>[6x]MKDILEKLEERRAQARLGGGEKRLEAQHKRGKLTARERIELLLDHGSFEEFDMFVQHRSTDFGMEKQKIPGDGVVTGWGTVNGRTVFLFSKDFTVFGGSSSEAHAAKIVKVQDMALKMRAPIIGIFDAGGARIQEGVAALGGHGEVFRRNVAASGVIPQISVIMGPCAGGDVYSPAMTDFIFMVRDTSYMFVTGPDVVKTVTNEVVTAEELGGAKVHTSKSSIADGSFENDVEAILQIRRLLDFLPANNIEGVPEIESFDDVNRLDKSLDTLIPDNPNKPYDMGELIRRVVDEGDFFEIQAAYARNIITGFGRVEGRTVGFVANQPLVLAGVLDSDASRKAARFVRFCNAFSIPIVTFVDVPGFLPGTAQEYGGLIKHGAKLLFAYSQATVPLVTIITRKAFGGAYIVMASKHVGADLNYAWPTAQIAVMGAKGAVEIIFRAEIGDADKVAERTKEYEDRFLSPFVAAERGYIDEVIMPHSTRKRIARAL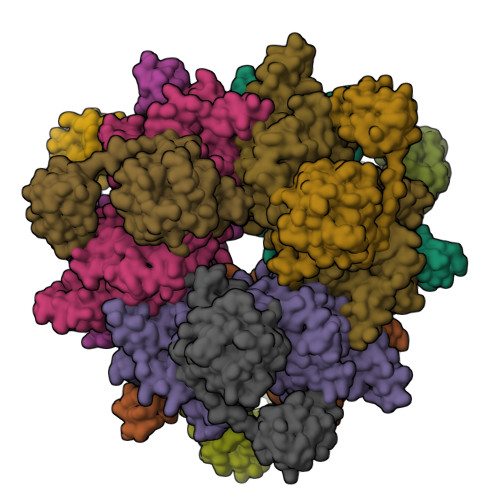GMLRTKEMEQPRKKHDNIPL;>[6x]MFDKILIANRGEIACRIIKTAQKMGIKTVAVYSDADRDAVHVAMADEAVHIGPAPAAQSYLLIEKIIDACKQTGAQAVHPGYGFLSERESFPKALAEAGIVFIGPNPGAIAAMGDKIESKKAAAAAEVSTVPGFLGVIESPEHAVTIADEIGYPVMIKASAGGGGKGMRIAESADEVAEGFARAKSEASSSFGDDRVFVEKFITDPRHIEIQVIGDKHGNVIYLGERECSIQRRNQKVIEEAPSPLLDEETRRKMGEQAVALAKAVNYDSAGTVEFVAGQDKSFYFLEMNTRLQVEHPVTEMITGLDLVELMIRVAAGEKLPLSQDQVKLDGWAVESRVYAEDPTRNFLPSIGRLTTYQPPEEGPLGGAIVRNDTGVEEGGEIAIHYDPMIAKLVTWAPTRLEAIEAQATALDAFAIEGIRHNIPFLATLMAHPRWRDGRLSTGFIKEEFPEGFIAPEPEGPVAHRLAAVAAAIDHKLNIRKRGISGQMRDPSLLTFQRERVVVLSGQRFNVTVDPDGDDLLVTFDDGTTAPVRSAWRPGAPVWSGTVGDQSVAIQVRPLLNGVFLQHAGAAAEARVFTRREAELADLMPVKENAGSGKQLLCPMPGLVKQIMVSEGQEVKNGEPLAIVEAMKMENVLRAERDGTISKIAAKEGDSLAVDAVILEFA>MSLASISPQGSMSLLSQLEIERLKASSNSQLYKLFRNCCLAVLNAGSHTDSSADIYDSYKDFEVNIIRRERGIKLELIEPPEEAFVDGEVIVGIRELLESVLRDILFTGERYSETDLEHADSATLTHVVFDILRNARTLRPQEEPNMVVCWGGHSINEIEYKYTKDVGYHIGLRGLNICTGCGPGAMKGPMKGATIGHAKQRVEGGRYLGLTEPGIIAAEPPNPIVNELVILPDIEKRLEAFVRCAHGIVIFPGGAGTAEELLYLLGILMHPDNQRQSLPVILTGPASSRDYFEALDEFIGATIGDEARQLYKIIIDDPAAVAQHMH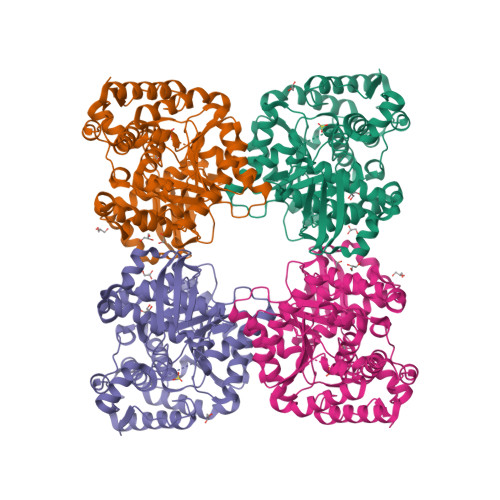AGMAAVKQYRRDSGDAYYFNWTLKINEEFQRPFSPTHENVAALNLHPDQPKERLAADLRRAFSAIVAGNVKDEGIRQIRKNGVFTIHGEQSLMKRLDELLRAFVEQGRMKLPGSVYNPCYKVITDEGHHHHHH[2x]4-[(1~{R})-1-[(2-methyl-5-phenyl-pyrazol-3-yl)carbonylamino]ethyl]benzoic acid | C20 H19 N3 O3 | 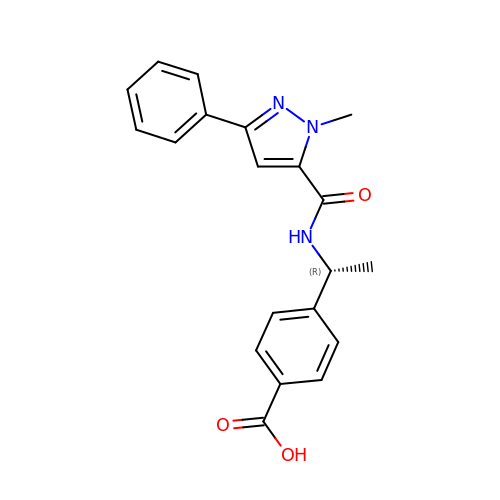ONVWOXXFKHGWTI-CYBMUJFWSA-N>[5x]GSHMGGVEVLEVKTGVDSITEVECFLTPEMGDPDEHLRGFSKSISISDTFESDSPNRDMLPCYSVARIPLPNLNEDLTCGNILMWEAVTLKTEVIGVTSLMNVHSNGQATHDNGAGKPVQGTSFHFFSVGGEALELQGVLFNYRTKYPDGTIFPKNATVQSQVMNTEHKAYLDKNKAYPVECWVPDPTRNENTRYFGTLTGGENVPPVLHITNTATTVLLDEFGVGPLCKGDNLYLSAVDVCGMF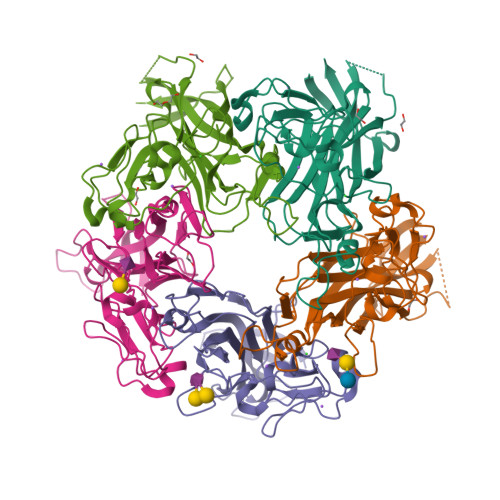TNRSGSQQWRGLSRYFKVQLRKRRVKN> FNWNKNQVIAHRGAWKKNNFPQNSIASLNEAVKLGCYGSEFDVWMTADHILVVNHDPEFQG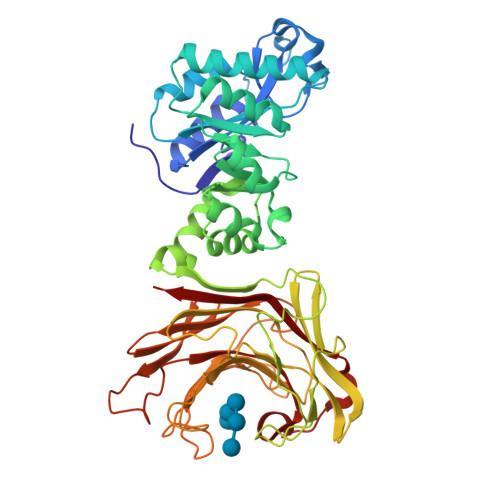LTIEKVNYADLLTKTMSNGEKIPTLEAYLLAGKKQKSTKLILEIKPSLISKERGIEVTNKCVEMVQKLKVTDWVEYISFDYDYCKRILTLLPNAKVAYLKGEVSAEQMKADKLTGVDYHYSVYQKDNWIENAQKLGLTVNAWTVNAVPEMQWLLAHNVDYITTNEPELLFDEIKKAPVAQGWKLKWADEFDNSGLPLNKNWGYDVGGRGWGNNELQYYTDADSANAIVKKGNLNIIALKAEKENRHYTSARLVTKNKFDFKYGRVEVRAMLPKGRGLWPAIWALPTDSKYGSWPKSGEIDIMEHVGFDPDSVHGTVHTEKFNHVIHTQVGKALKVNNPYTEYHIYAIEWFTDHIDFFIDDQKYLTFKNTQKGSGDWPFDQNFHILNLAVGGNWGGKKGVDDAIFPATMKVDYVRVFQK>NQFYSVEVGDSTFTVLKRYQNLKPIGSGAQGIVCAAYDAVLDRNVAIKKLSRPFQ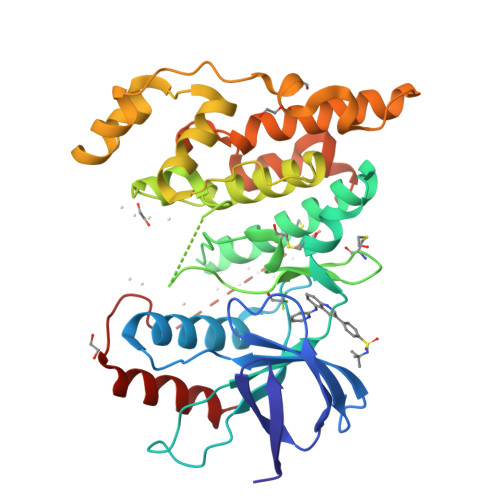NQTHAKRAYRELVLMKCVNHKNIISLLNVFTPQKTLEEFQDVYLVMELMDANLCQVIQMELDHERMSYLLYQMLCGIKHLHSAGIIHRDLKPSNIVVKSDCTLKILDFGLARTAGTSFMMTPYVVTRYYRAPEVILGMGYKENVDIWSVGCIMGEMVRHKILFPGRDYIDQWNKVIEQLGTPCPEFMKKLQPTVRNYVENRPKYAGLTFPKLFPDSLFPADSEHNKLKASQARDLLSKMLVIDPAKRISVDDALQHPYINVWYDPAEVEAPPPQIYDKQLDEREHTIEEWKELIYKEVMNS[2x]Olfactomedins comprise a large protein family (PFAM: PF02191) with seven phylogenetic branches. These multidomain proteins contain a ~30 kDa olfactomedin (OLF) domain and are predominantly expressed extracellularly in a variety of tissues of multicellular organisms, particularly in vertebrates as well as selected invertebrates. Here we present biophysical, biochemical, and structural characterization of the OLF domain of a second glio-OLF, that from M. musculus (94% identical to R. norvegicus), and H. sapiens noelin/pancortin/olfm1/hOlfA (npoh-OLF), which are both neuronal OLFs, but from different phylogenetic subfamilies. The OLF domain propeller blades are arranged radially around a central hydrophilic cavity.

For npoh-OLF, the point mutation C221G, before the start of the structural OLF domain, increased yields sufficient for crystallization (not shown). The 2.1 Å resolution structure npoh-OLF(C221G), and the 2.05 Å resolution structure of glio-OLF were solved by molecular replacement using search models derived from myoc-OLF and npoh-OLF, respectively. Npoh-OLF exhibits the expected OLF five-bladed β-propeller architecture with a short α-helix; no major conformational changes are seen between our mouse glio-OLF structure and the previously reported rat glio-OLF. Npoh-OLF has a clasp that extends longer than that of the other OLFs because it forms a crystal contact with the outermost strand of blade A from a neighboring molecule. Similarly, for npoh-OLF, Ca2+, but not Mg2+ or K+, confers thermal stability, and the Ca2+ ion is resistant to chelation by Quin-2, except under denaturing conditions. An analogous pair, Trp 349/Tyr 418, is found within npoh-OLF, and in the structure appears to be in a conformation that seals off the cavity. Myoc-OLF variants K423E and Y371D are associated with severe cases of glaucoma, and K423E is one of the least stable variants, supporting the importance of this feature in maintaining the structural integrity of the domain. In npoh-OLF the corresponding residues are Lys 399 and Tyr 347 and the interaction is part of an extended hydrogen-bonding network; the hydroxyl group of the Tyr stabilizes the carboxylate side chain of Asp 356, which helps position this residue for coordination to Ca2+ (and see above). For npoh-OLF, 18 of 20 total Arg and Lys residues are solvent exposed, with a large positive region concentrated at the top face of blades A and B and extending into two small positive patches involving Arg 400 of the short helical turn and Lys 423 of the loop between strands D-16 and D-17.

> LRAGMQKLACGKLTGISDPVTVKTSGSRFGSWMTDPLAPEGDNRVWYMDGYHNNRFVREYKSMVDFMNTDNFTSHRLPHPWSGTGQVVYNGSIYFNKFQSHIIIRFDLKTETILKTRSLDYAGYNNMYHYAWGGHSDIDLMVDESGLWAVYATNQNAGNIVVSRLDPVSLQTLQTWNTSYPKRSAGEAFIICGTLYVTNGYSGGTKVHYAYQTNASTYEYIDIPFQNKYSHISMLDYNPKDRALYAWNNGHQILYNVTLFHVIRSDEL> GSGEVNLLDSKTIQGELGWISYPSHGWEEISGVDEHYTPIRTYQVCNVMDHSQNNWLRTNWVPRNSAQKIYVELKFTLRDCNSIPLVLGTCKETFNLYYMESDDDHGVKFREHQFTKIDTIAADESFTQMDLGDRILKLNTEIREVGPVNKKGFYLAFQDVGACVALVSVRVYFKK;> GSGAVADRYAVYWNSSNPRFQRGDYHIDVCINDYLDVFCPHYEDSVPEDKTERYVLYMVNFDGYSACDHTSKGFKRWECNRPHSPNGPLKFSEKFQLFTPFSLGFEFRPGREYFYISSAIPDNGRRSCLKLKVFVRPTNSCMK

The Eph receptor tyrosine kinase family regulates a variety of physiological processes in the developing and adult organism, ranging from tissue patterning and angiogenesis to glucose homeostasis and bone remodeling, while its dysregulation has been implicated in diseases such as cancer. The ligand-binding domain (LBD) of the Eph receptors comprises approximately 200 amino acids at the N-terminus of the extracellular region and is followed by a cysteine-rich region and two fibronectin III repeats. Binding to ephrin ligands on opposing cells causes the Eph receptors to cluster, which involves only a subtle conformational rearrangement of the extracellular region and the formation of receptor-receptor interfaces. We report the structure of the human EphA3 LBD in complex with its preferred ligand, ephrin-A5, which reveals a large interface with an extensive network of contacts.

The human EphA3 LBD was crystallized in complex with the receptor-binding domain of the human ephrin-A5 ligand and the structure was determined to 2.26 Å resolution with an Rcryst/Rfree of 0.19/0.21, bond/angle residual mean square deviations (RMSD) of 0.004 Å/0.78°, and no Ramachandran outliers. The crystals contained one heterodimer in the asymmetric unit with a well-ordered interface. A notable difference is that ephrin-A5 is more tilted when bound to EphA3 compared to other EphA/ephrin-A complexes such as EphA2/ephrin-A5. Thus, EphA3 binds ephrin-A5 in a manner similar to EphA4 but different from EphA2 and EphB2. In contrast, the pronounced tilt of ephrin-A5 in our structure brings the ephrin ligand closer to the ABR loop (R indicates the EphA3 receptor and L indicates the Ephrin A5 ligand) and burying a larger surface area (as calculated with Protein Interfaces, Surfaces and Assemblies (PISA) and Shape Correlation statistics (SC) software). The EphA3 C strand lining the bottom half of the ephrin-binding pocket is remarkably twisted, which enables extensive contacts with ephrin-A5 residues outside of the ephrin GH loop. One consequence of this larger twist in EphA3 is that residues S49-V58 from the C strand are brought into contact with ephrin-A5 residues located below the ephrin-binding pocket. Ephrin-A5 inserts its GH loop into the well conserved ephrin-binding pocket of EphA3. Nine residues of the ephrin GH loop penetrate the ephrin-binding pocket of EphA3 forming contacts with seventeen residues of the receptor, and six of the nine ephrin-A5 residues interact with EphA3 through salt bridges and hydrogen bonds, consistent with tight binding. The strategic placement of L111R, which caps the ephrin-binding pocket, is unique because in all other Eph receptor crystal structures a proline occupies this position near the edge of the ephrin-binding pocket, leaving the pocket open.5-CYCLOHEXYL-1-PENTYL-BETA-D-MALTOSIDE | C23 H42 O11 | 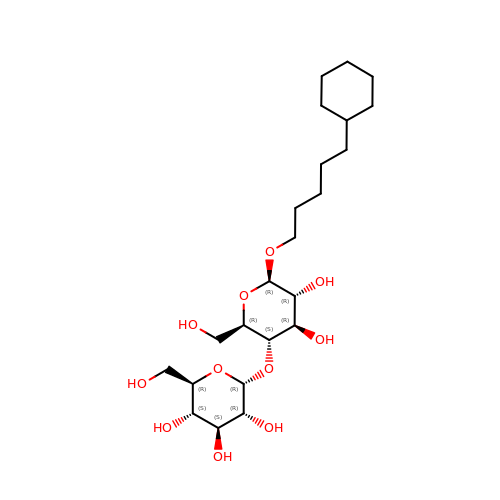RVTGFZGNOSKUDA-ZNGNCRBCSA-N>AEGQTNADDTLVVEASTPSLYAPQQSADPKFSRPVADTTRTMTVISEQVIKDQGATNLTDALKNVPGVGAFFAGENGNSTTGDAIYMRGADTSNSIYIDGIRDIGSVSRDTFNTEQVEVIKGPSGTDYGRSAPTGSINMISKQPRNDSGIDASASIGSAWFRRGTLDVNQVIGDTTAVRLNVMGEKTHDAGRDKVKNERYGVAPSVAFGLGTANRLYLNYLHVTQHNTPDGGIPTIGLPGYSAPSAGTAALNHSGKVDTHNFYGTDSDYDDSTTDTATMRFEHDINDNTTIRNTTRWSRVKQDYLMTAIMGGASNITQPTSDVNSWTWSRTANTKDVSNKILTNQTNLTSTFYTGSIGHDVSTGVEFTRETQTNYGVNPVTLPAVNIYHPDSSIHPGGLTRNGANANGQTDTFAIYAFDTLQITRDFELNGGIRLDNYHTEYDSATACGGSGRGAITCPTGVAKGSPVTTVDTAKSGNLMNWKAGALYHLTENGNVYINYAVSQQPPGGNNFALAQSGSGNSANRTDFKPQKANTSEIGTKWQVLDKRLLLTAALFRTDIENEVEQNDDGTYSQYGKKRVEGYEISVAGNITPAWQVIGGYTQQKATIKNGKDVAQDGSSSLPYTPEHAFTLWSQYQATDDISVGAGARYIGSMHKGSDGAVGTPAFTEGYWVADAKLGYRVNRNLDFQLNVYNLFDTDYVASINKSGYRYHPGEPRTFLLTANMHF[2x]

The ferric iron uptake (Fiu) transporter is a TBDT responsible for import of molecules containing the catecholate functional group. Members of the TonB-dependent transporter (TBDT)3 family drive transport of their substrates through interaction with the energy-transducing protein TonB. The structure of Fiu consists of a 22-stranded transmembrane β-barrel characteristic of the TBDT superfamily, with a number of extended extracellular loops that might serve in the initial steps of substrate binding. In addition to its role in iron uptake, Fiu has also been shown to be important for sensitivity to antimicrobials that share the common feature of a catecholate functional group or the analogous dihydroxypyridine moiety.

The structure of Fiu was solved in three different crystal forms, revealing Fiu in two distinct states. In contrast, in crystal state 2, the entire polypeptide chain (amino acids 50–760) C-terminal of the TonB box (which is disordered in both crystal forms) could be modeled into the available electron density. The disorder of the plug domain loop in crystal state 1 opens a large cavity in the interior of Fiu to the external environment, whereas, in crystal state 2, this cavity is present but occluded in the lumen of the Fiu barrel. In crystal state 2, removal of the labile subdomain opens the internal cavity of Fiu to the periplasm, but because of the presence of the plug loop, this does not create a membrane-spanning channel. For the first run, the entire extracellular portion of closed Fiu (crystal state 2) was defined as the search area. In this experiment, the majority of the solutions placed Fe–DHB in the internal chamber of Fiu, with the third most favored solution positioning Fe–DHB in the extracellular cavity of the protein. Although the internal cavity would be inaccessible to Fe–DHB in the closed state, because of the fully ordered plug loop, it would be accessible in state 1, as this loop is disordered. Specifically, the external plug loop of Fiu in our structures selectively gates a large cavity in the lumen of the transporter.>[4x]MHAALTPLTNKYRFIDVQPLTGVLGAEITGVDLREPLDDSTWNEILDAFHTYQVIYFPGQAITNEQHIAFSRRFGPVDPVPILKSIEGYPEVQMIRREANESSRFIGDDWHTDSTFLDAPPAAVVMRAIEVPEYGGDTGFLSMYSAWETLSPT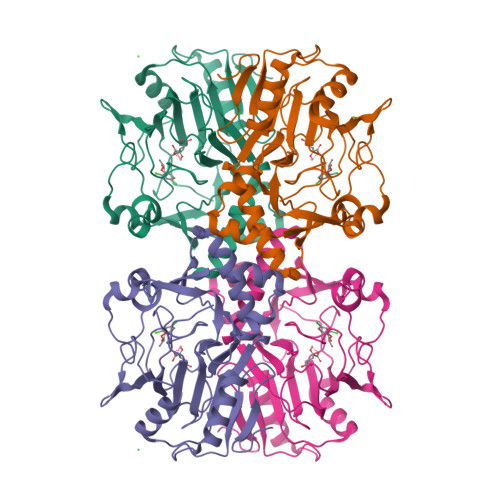MQATIEGLNVVHSATKVFGSLYQATNWRFSNTSVKVMDVDAGDRETVHPLVVTHPVTGRRALYCNQVYCQKIQGMTDAESKSLLQFLYEHATKFDFTCRVRWKKDQVLVWDNLCTMHRAVPDYAGKFRYLTRTTVAGDKPSR>[2x]GAHMSYSYDAPSDFINFSSKQKNEESKKRQWALEDFEIGRPLGKGKFGNVYLAREKQSKFILALKVL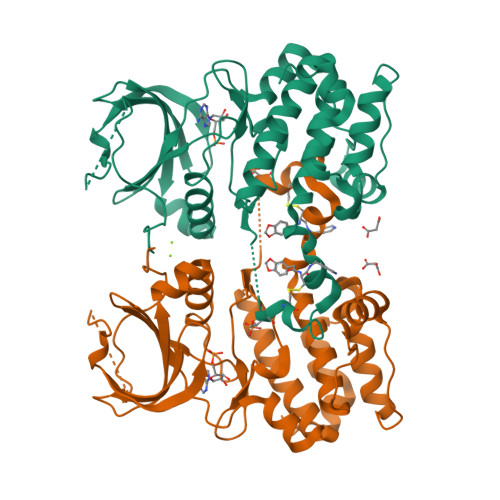FKAQLEKAGVEHQLRREVEIQSHLRHPNILRLYGYFHDATRVYLILEYAPLGTVYRELQKLSKFDEQRTATYITELANALSYCHSKRVIHRDIKPENLLLGSAGELKIADFGWSVHAPSSRRTTLCGTLDYLPPEMIEGRMHDEKVDLWSLGVLCYEFLVGKPPFEANTYQETYKRISRVEFTFPDFVTEGARDLISRLLKHNPSQRPMLREVLEHPWITANSSK> GSQIPASEQETLVRPKPLL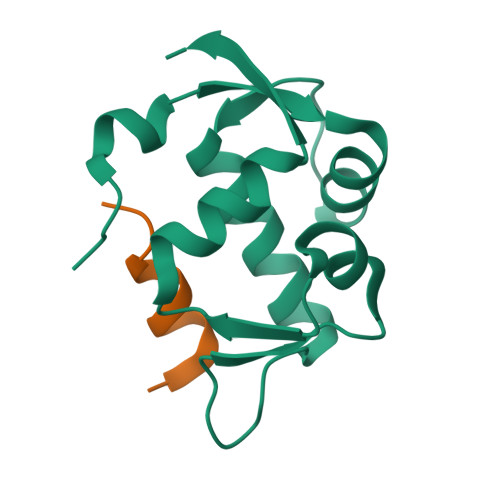LKLLKSVGAQKDTYTMKEVLFYLGQYIMTKRLYDEKQQHIVYCSNDLLGDLFGVPSFSVKEHRKIYTMIYRNLVVVNQQESSDSGTSVSEN;> LTFEHWWAQLTS>[4x]VAQISPQYPMFTVPLPIPPVKQPRLTVTNPVNGQEIWYYEVEIKPFTHQVYPDLGSADLVGYDGMSPGPTFQVPRGVETVVRFINNAEAPNSVHLHGSFSRAAFDGWAEDITEPGSFKDYYYPNRQSARTLWYHDHAMHITAENAYRGQAGLYMLTDPAEDALNLPSGYGEFDIPMILTSKQYTANGNLVTTNGELNSFWGDVIHVNGQPWPFKNVEPRKYRFRFLDAAVSRSFGLYFADTDAIDTRLPFKVIASDSGLLEHPADTSLLYISMAERYEVVFDFSDYAGKTIELRNLGGSIGGIGTDTDYDNTDKVMRFVVADDTTQPDTSVVPANLRDVPFPSPTTNTPRQFRFGRTGPTWTINGVAFADVQNRLLANVPVGTVERWELINAGNGWTHPIHIHLVDFKVISRTSGNNARTVMPYESGLKDVVWLGRRETVVVEAH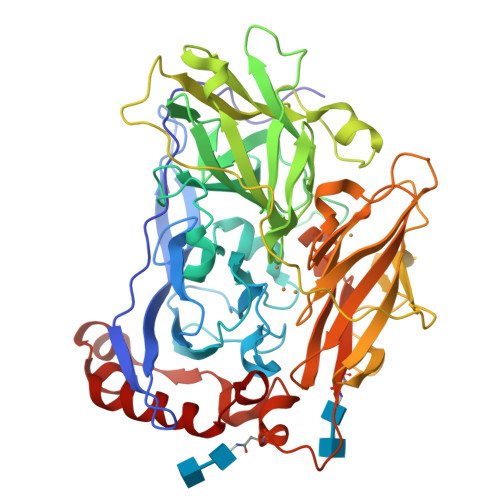YAPFPGVYMFHCHNLIHEDHDMMAAFNATVLPDYGYNATVFVDPMEELWQARPYELGEFQAQSGQFSVQAVTERIQTMAEYRPYAAADE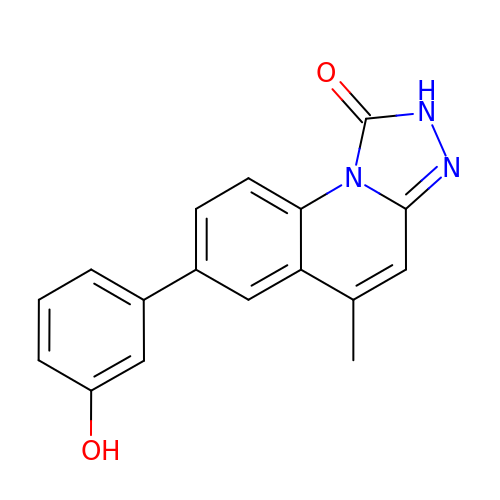7-(3-hydroxyphenyl)-5-methyl[1,2,4]triazolo[4,3-a]quinolin-1(2H)-one | C17 H13 N3 O2 | UWWPFTOELGGCIL-UHFFFAOYSA-N In this study, we have identified a new specific binding partner of M. smegmatis σA, MoaB2, that appears not to interact with alternative σ factors. MoaB2 is a 17.9 kDa (pI 4.17) protein of unknown function. Functional experiments then showed that MoaB2 inhibits σA-dependent (but not σB-dependent) transcription and may increase the stability of σA in the cell. Likewise, the role of M. smegmatis MoaB2 in Moco biosynthesis is unlikely, especially when M. smegmatis MoaB2 contains serine at the respective position (Ser51).

In the crystal, MoaB2 was present as a hexamer. In crystal, the M. smegmatis MoaB2 hexamer forms the asymmetric unit. Each subunit of the hexamer exhibited a weak or missing electron density for the N-terminal residues 1–7, the C-terminal His-tag, and linker residues from the plasmid. The structure of each subunit of M. smegmatis MoaB2 is composed of a central β-sheet that is slightly curved and is surrounded by six α-helices and one 310 helix. The β-sheet is made up of five parallel strands (β1–β4 and β6) and one antiparallel strand (β5), which are located between the inner β4 strand and the adjacent β6 strand. The overall architecture of the protein subunit is similar to other known molybdopterin (MPT)-adenylyl-transferase enzymes. The hexamers are made up of two trimers (chains ABC and DEF) making contacts through mostly hydrophobic and salt-bridge interactions at the interface between the subunits. Assembly of subunits into trimers within the hexamer is strengthened through several hydrogen bonds between Arg95 and Arg120 of one monomer and Val79, Thr80, and Pro81 of another monomer. Residues Leu31, Glu34, and Glu38 in α4-helix and Arg138 and Arg142 in α7-helix form the central core of the trimer-trimer interface. Calculations using the Adaptive Poisson-Boltzmann Solver showed that the electrostatic potential on the surface of M. smegmatis MoaB2 is prominently negative.

>MEQPGELVGRALVIVVDDRTAHGEEDHSGPLVTELLGEAGFVVDGVVVVASDEVEIRNALNTAVIGGVDLVVSVGGTGVTPRDVTPEATRELLDRELLGISEALRASGLAAGIVDAGLSRGLAGISGSTLVVNIAGSRAAVRDGMATLGPLAVQIIGQLSSLEILEHHHHHH[6x]> GPKKTDPELAEKINEMLDVILEYKNEDGELIADVFQTLPTRKELPDYYQVISKPMDFDRINKKIETGRYTVMEELNDDMNLLVNNAQTYNEEGSEIYVSSETIGKLWKEQYDKFMNPPKPVEE;> ARKSTGGKAPRKQL

SMARCA4/BRG1 is an essential catalytic core subunit of the roughly two-megadalton Switch/Sucrose Nonfermenting (SWI/SNF) multiprotein complex, which uses the energy of ATP hydrolysis to remodel chromatin by perturbing interactions between histone core particles and DNA. SMARCA4 can remodel nucleosomal substrates by itself in vitro and is functionally and structurally conserved among eukaryotes. This remodeling enzyme possesses intrinsic ATPase and helicase activity and has a C-terminal BD motif capable of recognizing lysine 14 acetylation on histone H3 (H3K14ac). Bromodomains (BD) are conserved reader modules that bind acetylated lysine residues on histones. We use the reference nematode Caenorhabditis elegans and its SMARCA4 ortholog (SWSN-4 or CeSMARCA4)—which is conserved among eukaryotes and constitutes the only SWI/SNF ATPase in the worm—as a model.

To understand how SMARCA4 interacts with modified histones, we determined the crystal structure of the C. elegans SMARCA4 BD (residues 1176–1296) in complex with an H37–20K14ac modified peptide at 1.29 Å resolution. The CeSMARCA4 BD exhibits the canonical fold of a left-handed bundle of four α-helices (αZ, αA, αB, αC) linked by one long (ZA) and two short (AB and BC) interhelical loops. Residues H313–17 of the modified histone peptide could be unequivocally traced in the electron density map. The histone peptide lysine acetylamide binds within the central, largely hydrophobic cavity, as observed for other BDs, including the recently reported family VIII, yeast RSC ScSth1 BD–H3K14ac complex. The acetyl carbonyl group of H3K14ac forms hydrogen bonds with the conserved Asn1263 residue and a water molecule that bridges to the conserved Tyr1220 residue. Site-directed mutations of Tyr1220Ala or Asn1263Ala in the CeSMARCA4 BD independently abolish binding to H3 N-terminal tails in vitro, as confirmed by ITC. The H3A15 sidechain packs adjacent to the BC loop, anchored by hydrogen bonds between the peptide main chain with the carbonyl δ1-oxygen of the conserved Asn1263 and the backbone amide of Glu1264 (Leu1573 in HsSMARCA4/2). The H3P16 cyclic sidechain packs closely with the Tyr1262 benzene ring (Phe1571 in HsSMARCA4/2). The H3R17 sidechain is tethered to the BD αB-helix and BC loop via hydrogen bonds between the sidechain nitrogen atoms and the main-chain Gln1260, Thr1261, and Asn1263 carbonyl groups—all conserved in HsSMARCA4/2. After refinement, the dominant rotamer (60% occupancy) forms a hydrogen bond with H3R17, while the secondary rotamer (40% occupancy) is oriented toward Tyr1270.> PTGLAADIRWTAYGVPHIRAKDERGLGYGIGYAYARDNACLLAEEIVTARGERARYFGSEGKSSAELDNLPSDIFYAWLNQPEALQAFWQAQTPAVRQLLEGYAAGFNRFLREADGKTTSCLGQPWLRAIATDDLLRLTRRLLVEGGVGQFADALVAAAPPGAEK;> SNAIAVGSERSADGKGMLLANPHFPWNGAMRFYQMHLTIPGRLDVMGASLPGLPVVNIGFSRHLAWTHTVDTSSHFTLYRLALDPKDPRRYLVDGRSLPLEEKSVAIEVRGADGKLSRVEHKVYQSIYGPLVVWPGKLDWNRSEAYALRDANLENTRVLQQWYSINQASDVADLRRRVEALQGIPWVNTLAADEQGNALYMNQSVVPYLKPELIPACAIPQLVAEGLPALQGQDSRCAWSRDPAAAQAGITPAAQLPVLLRRDFVQNSNDSAWLTNPASPLQGFSPLVSQEKPIGPRARYALSRLQGKQPLEAKTLEEMVTANHVFSADQVLPDLLRLCRDNQGEKSLARACAALAQWDRGANLDSGSGFVYFQRFMQRFAELDGAWKEPFDAQRPLDTPQGIALDRPQVATQVRQALADAAAEVEKSGIPDGARWGDLQVSTRGQERIAIPGGDGHFGVYNAIQSVRKGDHLEVVGGTSYIQLVTFPEEGPKARGLLAFSQSSD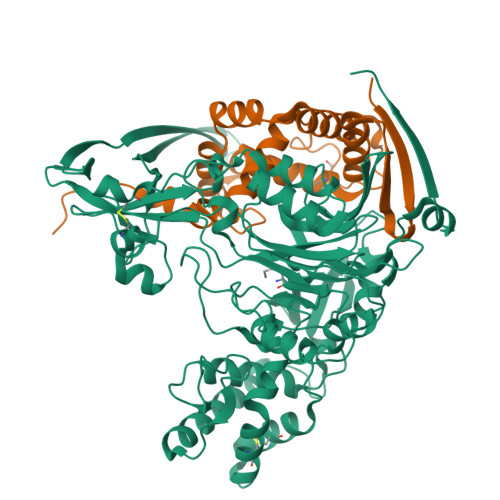PRSPHYRDQTELFSRQQWQTLPFSDRQIDADPQLQRLSIREAA>MIQNHIKNMTPEICKASRALVNLTQKEL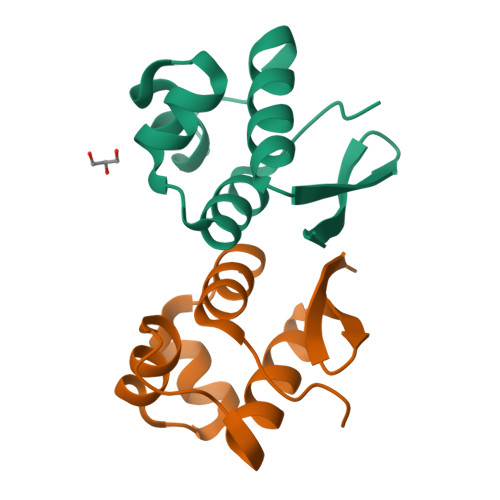ALMAGIATPTIADFERGARKPHGNNLRSIIIAFENKGLDFVEEGGEIIGIFIRRKNVRAEESIDLSGHGSH[2x]> MTQCASRRKSTPNRAILGAFASARGTRWVATIAG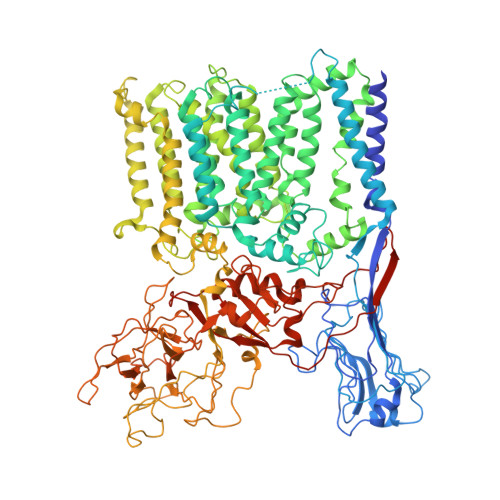LIGFVLSVATPLLPVVQTTAMLDWPQRGQLGSVTAPLISLTPVDFTATVPCDVVRAMPPAGGVVLGTAPKQGKDANLQALFVVVSAQRVDVTDRNVVILSVPREQVTSPQCQRIEVTSTHAGTFANFVGLKDPSGAPLRSGFPDPNLRPQIVGVFTDLTGPAPPGLAVSATIDTRFSTRPTTLKLLAIIGAIVATVVALIALWRLDQLDGRGSIAQLLLRPFRPASSPGGMRRLIPASWRTFTLTDAVVIFGFLLWHVIGANSSDDGYILGMARVADHAGYMSNYFRWFGSPEDPFGWYYNLLALMTHVSDASLWMRLPDLAAGLVCWLLLSREVLPRLGPAVEASKPAYWAAAMVLLTAWMPFNNGLRPEGIIALGSLVTYVLIERSMRYSRLTPAALAVVTAAFTLGVQPTGLIAVAALVAGGRPMLRILVRRHRLVGTLPLVSPMLAAGTVILTVVFADQTLSTVLEATRVRAKIGPSQAWYTENLRYYYLILPTVDGSLSRRFGFLITALCLFTAVFIMLRRKRIPSVARGPAWRLMGVIFGTMFFLMFTPTKWVHHFGLFAAVGAAMAALTTVLVSPSVLRWSRNRMAFLAALFFLLALCWATTNGWWYVSSYGVPFNSAMPKIDGITVSTIFFALFAIAAGYAAWLHFAPRGAGEGRLIRALTTAPVPIVAGFMAAVFVASMVAGIVRQYPTYSNGWSNVRAFVGGCGLADDVLVEPDTNAGFMKPLDGDSGSWGPLGPLGGVNPVGFTPNGVPEHTVAEAIVMKPNQPGTDYDWDAPTKLTSPGINGSTVPLPYGLDPARVPLAGTYTTGAQQQSTLVSAWYLLPKPDDGHPLVVVTAAGKIAGNSVLHGYTPGQTVVLEYAMPGPGALVPAGRMVPDDLYGEQPKAWRNLRFARAKMPADAVAVRVVAEDLSLTPEDWIAVTPPRVPDLRSLQEYVGSTQPVLLDWAVGLAFPCQQPMLHANGIAEIPKFRITPDYSAKKLDTDTWEDGTNGGLLGITDLLLRAHVMATYLSRDWARDWGSLRKFDTLVDAPPAQLELGTATRSGLWSPGKIRIGPHLGGIKAFHHHHHHHHHH threonylcarbamoyladenylate | C15 H21 N6 O11 P | 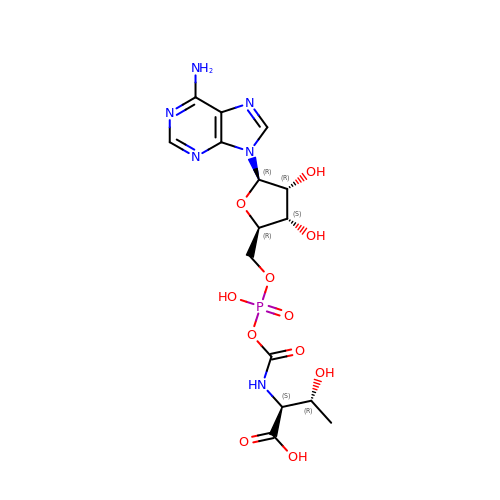GHLUPQUHEIJRCU-DWVDDHQFSA-N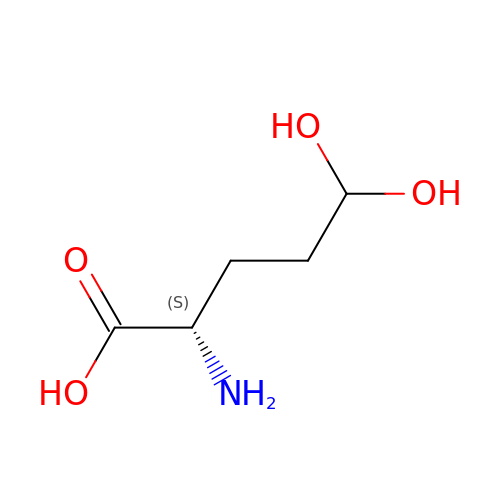5,5-dihydroxy-L-norvaline | C5 H11 N O4 | FIKXYBCGRJPSSD-VKHMYHEASA-N>SNAMDKNIIIGAMTALITPFKNGKVDEQSYARLIKRQIENGIDAVVPVGTTGESATLTHEEHRTCIEIAVETCKGTKVKVLAGAGSNATHEAVGLAKFAKEHGADGILSVA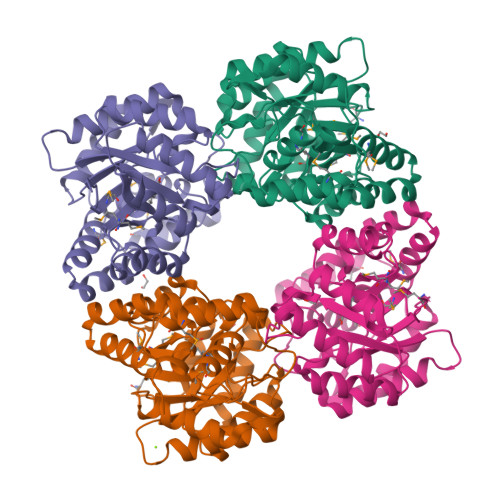PYYNKPTQQGLYEHYKAIAQSVDIPVLLYNVPGRTGCEISTDTIIKLFRDCENIYGVKEASGNIDKCVDLLAHEPRMMLISGEDAINYPILSNGGKGVISVTSNLLPDMISALTHFALDENYKEAKKINDELYNINKILFCESNPIPIKTAMYLAGLIESLEFRLPLCSPSKENFAKIEEVMKKYKIKGF[4x]> MTENIISVDHLTYQYDENQAPALTDVSFTVHAGEWLAIVGHNGSGKSTLAKSLDGLLPFTQGSVTVGGITLTPETVWQVREQIGMIFQNPDNQFVGATVEDDVAFGLENR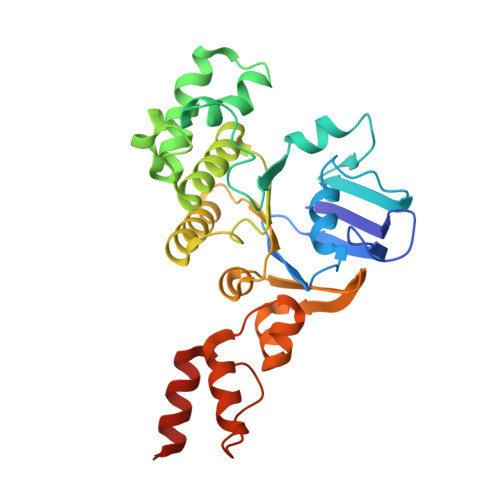QISRDEMVPRVQAALAQVGMTSFAQREPSSLSGGQKQRVALAGIVAIAPKILILDEATSMLDPQGRIEMLAIVRQLRQQQNLTVISITHDIDEAASADRVLVIDDGRLVDEAVPSQIFERGTQLVEMGLDLPFTEKLKAALRQRGITPPTTYQTAAEMEEWLWQSLSNT> MPSIKPPLIAVELENPMLGEVIDLEETKAIVIAAYENKALALLFDYYTGEIKQINRQGNTYKIAVSEDYIGGIFNGFGEPIKGPKPYPEDYRDINGLAINPYARKVPNEILYTGISSIDVAHPLLKGQKIAIFSPPGLPMERLALQIA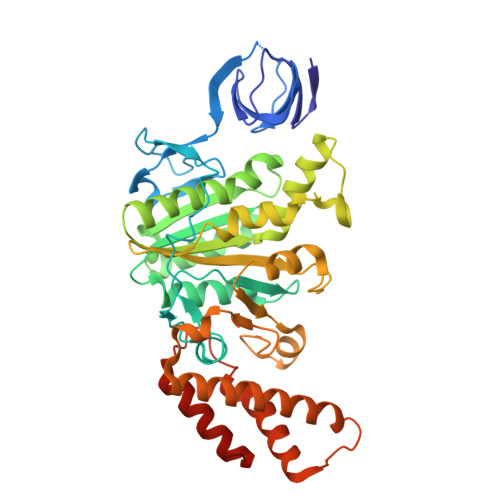RNVAKDKTIIFAAIGVPSDIYKMFIDEFINTKAIMNSAIFISKADSSPIEKIYTPRVALTLAEYLAFEKNRDVLVLMLDMTNYADALREISTLRKEIPSRRGYPAYLYTDLASIYERSGLTSKGSITLIPMLTMPGNDITHVVPDLTGYITEGQYVLSQDLHSKNIYPPIDLLKSLSRLAKNGMSKKHKKYADILIKSYAKGLEARDIATIVGEDSLSKEDKAYLKFAELVEKEFIKQDYYEYRSIEKSFEIIDSILSQSGLPYSPIQ>MAMTLRDMDAVRPVNREAVDRHKARMRDEVRAFRLRELRAAQSLTQVQVAALAHIRQSRVSSIENGDIGSAQVNTLRKYVSAL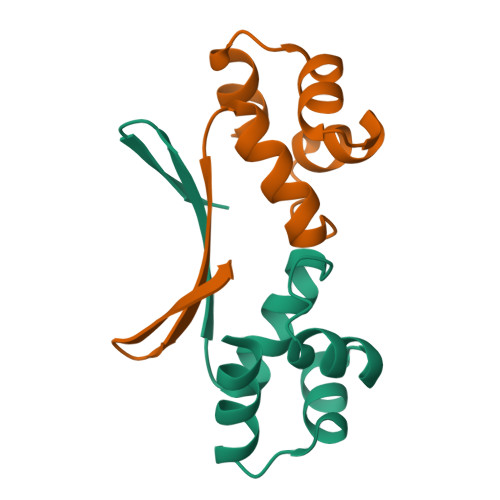GGELDITVRLGDETFTLA[4x]N,N-dibenzyl-1-hydroxy-1,3-dihydrobenzo[c][1,2]oxaborole-6-carboxamide 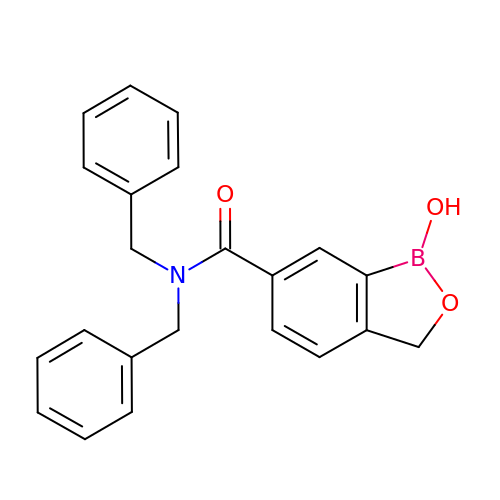| C22 H20 B N O3 | KHPGSFWNOIQUOW-UHFFFAOYSA-N Momelotinib | C23 H22 N6 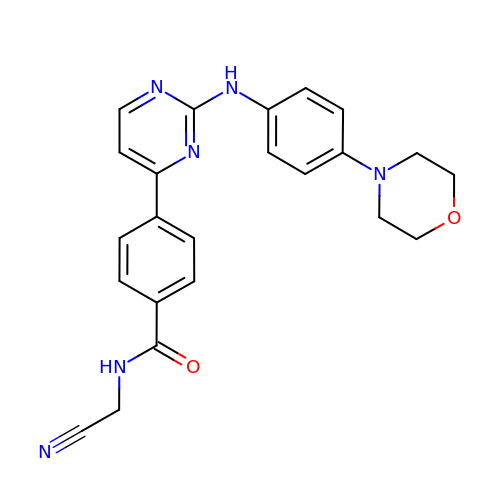O2 | ZVHNDZWQTBEVRY-UHFFFAOYSA-N> SMAATAAEAVASGSGEPREEAGALGPAWDESQLRSYSFPTRPIPRLSQSDPRAEELIENEEPVVLTDTNLVYPALKWDLEYLQENIGNGDFSVYSASTHKFLYYDEKKMANFQNFKPRSNREEMKFHEFVEKLQDIQQRGGEERLYLQQTLNDTVGRKIVMDFLGFNWNWINKQQGKRGWGQLTSNLLLIGMEGNVTPAHYDEQQNFFAQIKGYKRCILFPPDQFECLYPYPVHHPCDRQSQVDFDNPDYERFPNFQNVVGY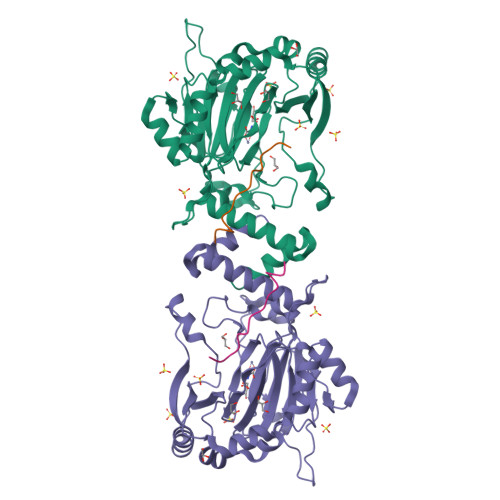ETVVGPGDVLYIPMYWWHHIESLLNGGITITVNFWYKGAPTPKRIEYPLKAHQKVAIMRNIEKMLGEALGNPQEVGPLLNTMIKGRYN;> GHTEIVKFLVQFGVNVNAADSDG>[3x]MATPHINAEMGDFADVVLMPGDPLRAKYIAETFLEDAREVNNVRGMLGFTGTYKGRKISVMGHGMGIPSCSIYTKELITDFGVKKIIRVGSCGAVLPHVKLRDVVIGMGACTDSKVNRIRFKDHDFAAIADFDMVRNAVDAAKALGIDARVGNLFSADLFYSPDGEMFDVMEKYGILGVEMEAAGIYGVAAEFGAKALTICTVSDHIRTHEQTTAAERQTTFNDMIKIALESVLLGDKE

PNP is a ubiquitous enzyme that reversibly converts purine nucleosides into nucleobases and α-pentose-1-phosphate, and is responsible for the regulation of nucleoside concentration within cells. The hexameric molecule of PNP from E. coli can be described as a trimer of dimers. The key role in the catalysis of natural enzyme substrates is played by Asp204, which is protonated, and by Arg217. Closing of the active site is a necessary step in catalysis; it brings Arg217 closer to Asp204 and enables the formation of a hydrogen bond between these residues, with deprotonation of Asp204 and protonation of N7 of the purine ring, which initiates catalysis.

In the WT PNP-N2,3-ε2APu and D204N-PNP-N2,3-ε2APu structures, the ligand is bound in all subunits, as the electron density in the appropriate region of the active site is in this case unambiguous. In both structures, there is one subunit in the closed (chain A) and two subunits in the open (chains B and C) active site conformations; thus, an active hexamer is composed of two asymmetric open–closed dimers (A-C, A’-C’) and one symmetric open–open dimer (B-B’). In all active sites, a phosphate ion (or a sulfate ion from the crystallization liquid) is bound in a typical position, at a hydrogen bond distance from Arg43* (from the neighboring subunit) and Arg87, while in the active sites with the closed conformation, also from Arg24. As there is no pentose in the N2,3-ε2APu molecule, in the case of the WT enzyme, this part of the active site is occupied by glycerol, which was used as a cryoprotectant. The orientation of N2,3-ε2APu in the active site cannot be determined unambiguously as, at this resolution, the electron density blob is symmetric. In the case of the WT PNP, the orientation differs in the closed and open active site conformations, whereas in the structure of the D204N enzyme, the orientation is identical in all active sites. In the closed active site conformation of the WT complex, N2,3-ε2APu can be modeled in an orientation where a hydrogen bond between Asp204 and N9 of the ligand is possible but, in this orientation, ribosylation would occur at N7. In the second possible orientation, C11 of the ligand is at a hydrogen bond distance from Asp204; thus, the hydrogen bond cannot be created, but ribosylation would occur on N2, which, indeed, predominantly occurs as described in Section 2.1.1. For the WT PNP-N2,3-ε2APu complex, in the active sites with the open conformation, the ligand is “flipped”. In one of them, a hydrogen bond can be created between Asp204 and N7 of the ligand; thus, ribosylation would occur on N9, while in the second one, N2 would be at a hydrogen-bonding distance but then ribosylation would occur on C11, which is impossible.> MRDPRYDILFEPVQIGPVTTKNRFYVVPHATAMGMTALEEMIAFRKARAEGGWGVVCLEETMIHETSDHAPLPDPRMYSDKYIEPLARVVAAVKEHGALAGVELAHAGASGPAIYHREHPLSPTTKYPHYFINPIAARTIDRQDIADFRRWYRDAALRAKRAGFDIVYVYCAHNLSLLQDFLDTRVNKRTDDYGGIFENRVRLLRETLSDVKDAVGDTCAVAVRFAVEDRRRQTNLTALEDGRRVVEALADVPDLWDVNVSDWAWDSGSSRF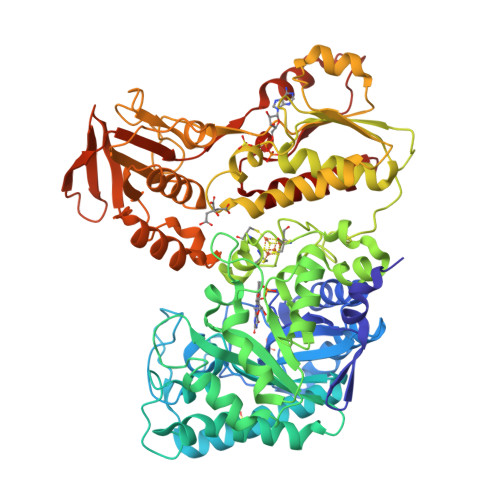FEEGQQEPFIDFVKKVTSKPVVGVGRFTSPDAMVSQIRRGVLDLIGAARPSIADPFLPNKIDAGLQDDIRECIGCNACTAEVMTSSRIRCTQNPSAGEEHVSGWHPEKVPPAHNSDASILVIGGGPAGLEAAHTLAKRGYQVSIADAGSEWGGRLVRERRLPRLSAWGRVVDYRVGQLQTMPNVSMYLDSPLGADDVAGFEADHVIVATGAKWRGEGVGRNHDEPIPGCDLPHVLTPEDILDGRLPEGGSVIVYDEDYYYMAAVVADRLARAGCKVTYVTTASDPSPWTHNTLEMVHVVNSMNEAGIEIVVGTAIASIGPSSVKVSRLLDGRENEMAADAVVLVTGQLSEDELYHQLIAKRDGGLLRSVERIGDCLGAGQIAQATYDGRKAGMRYGTSVE> AAFTQAPMLEQNKQLPPVDQRLPEKPLVIKPIASNGVYGGTLRTVMRGNADGNGILRTIGPQGLTHWTQDIQTVEPYVAESYTVSPDAMEYTFKLRKGMKWSDGTPFTADDIVFAMNDVVLNKEMFPQTPSAYLVGGKAPKVSKVDDYTVKFEFPAANLSFPETLATPLGQHPTLYQKKYCSQFHPAYNKNVQAEFTKANVKDWPSLMRAKCSDIELPSRWSSTERPSIDPWLIKEPYGGAVTRVVMERNPFYWQVDPTGKQLPYVDRIQYAVVSDLQAIILAATNGQYDIEARLLGSDVTSRPLMLKNQQKGGYKVFGQTSANANAAGLWLNQTTKNEKLRKYMTQHDFRQALSLAMDRDEINKVAWLGQAAPWQSGPFKESKWYNEKLATQYLKLDLAQANQILDRLGLTKRDSDGYRTYPDGGRVSLDAIVMIDRQAMVQTLELIRRQWQKAGVELVIKGSERSLFYNRATANDYDISIDVFPGGLDATLNPRAYVAVHPLESRMSLEWAKWYLSGGKQGIEPNESMKKRMALYDQFVAAKTQSQALSLFKQILQISADEFEVIGTVRPAVISSLHSLKLQNVNEKMPFGWPYATPSLSLPQQWYFSKLEHHHHHH

SPH1118 has been identified as a pectin-binding protein involved in both pectin chemotaxis and assimilation. SPH1118 shows high homology with the solute-binding protein (SBP) associated with the bacterial ABC transporter. SPH1118 consisted of two domains with a large cleft between the domains and substrates bound to positively charged and aromatic residues in the cleft through hydrogen bond and stacking interactions. Here we show tertiary structures of SPH1118 with six different conformations as determined by X-ray crystallography.

Interestingly, SPH1118 showed three conformations [SPH1118 (open form), SPH1118 (full open form), and SPH1118 (closed form)] even in the substrate-free state. These conformations were probably present in equilibrium in solution. The crystallization conditions of SPH1118 (open form), SPH1118 (full open form), and SPH1118 (closed form) contained the substrates (ΔtriGalUA or sodium PG). However, no substrates were bound to SPH1118 in these structures. The crystal structures of SPH1118 (full open form) and SPH1118 (closed form) were obtained only under crystallization conditions in the presence of sodium PG. Compared to the C terminal domain of SPH1118 (full open form), those of SPH1118 (open form) and SPH1118 (closed form) were closed by 18.9° and 34.2°, respectively, suggesting that the domain of SPH1118 was flexibly opened and closed even in the substrate-free state. SPH1118 (full open form) opened the domains more than SPH1118 (open form), thereby increasing the surface area exposed to the solvent and possibly accommodating the polysaccharide more efficiently.>[4x]GAHMSGRMTDDKDVLRDVWFGRIPTCFTLYQDEITEREAEPYYLLLPRVSYLTLVTDKVKKHFQKVMRQEDISEIWFEYEGTPLKWHYPIGLLFDLLAS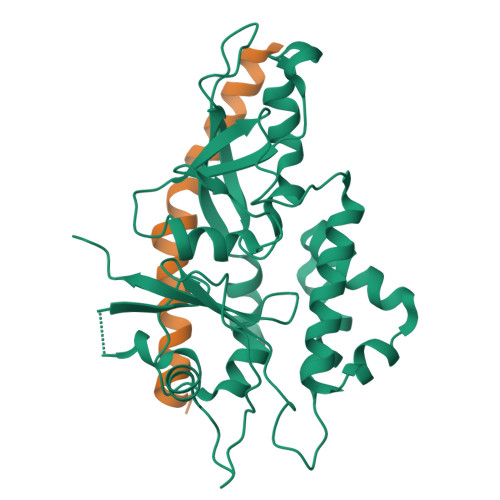SSALPWNITVHFKSFPEKDLLHCPSKDAIEAHFMSCMKEADALKHKSQVINEMQKKDHKQLWMGLQNDRFDQFWAINRKLMEYPAEENGFRYIPFRIYQTTTERPFIQKLFRPVAADGQLHTLGDLLKEVCPSAIDPEDGEKKNQVMIHGIEPMLETPLQWLSEHLSYPDNFLHISIIPQPTD;>[4x]GGGRPRWKRHISEQLRRRDRLQRQAFEEIILQYNKLLEKSDLHSVLAQKLQAEKHDVPNRHEISPGHDGTWNDNQLQEMAQLRIKHQEELTELHKKRGELAQLVIDLNNQMQRKDREMQMNEAKIAECLQTISDLETECLDLRTKLCDLERANQTLKDEYDALQITFTALEGKLRKTTEENQELVTRWMAEKAQEANRLNAENEKDSRRRQARLQKELAEAAKEPLPVEQDDDIEVIVDETSDHTEETSPVRAISRAATKRLSQPAGGLLDSITNIFGRRSVSSFPVPQDNVDTHPGSGKE>[4x]MGHHHHHHAWNVYAYPKSEKERVPETTKEAYHFVLVPEELDNDYWRLVEKGAKAAAKELGVDLEYIGPRQANIDEHLRILKKAAAAKVDGIITQGLTEAEFVPVINEITDKNIPVVTIDTDAPTSRRVAYVGTDNYYAGFLAGRALAEDTKGKATVAIITGSLTAAHQQLRVRGFEDAVRQEKGIRIVAIEESHITRVQAAEKAYTILKKHPDVNAFYGTSALDAI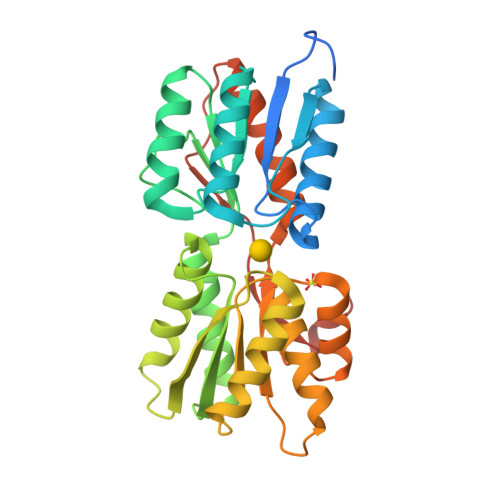GVAKVVEQFHREQKTYIIGFDTLPETIRYLQKGTIAATVVQEPYEMGYKAVKMMAEIVAGKDVPVVTNTETKVIRKKDLPLRPARNYEVNTP>[2x]EIPLKYGATNEGKRQDPAMQKFRDNRLGAFIHWGLYAIPGGEWNGKVYGGAAEWLKSWAKVPADEWLKLMDQWNPTKFDAKKWAKMAKEM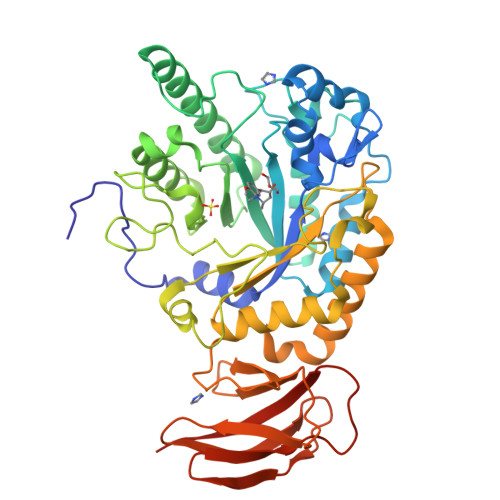GTKYVKITTKHHEGFCLWPSKYTKYTVANTPYKRDILGELVKAYNDEGIDVHFYFSVMDWSNPDYRYDIKSKEDSIAFSRFLEFTDNQLKELATRYPTVKDFWFDGTWDASVKKNGWWTAHAEQMLKELVPGVAINSRLRADDKGKRHFDSNGRLMGDYESGYERRLPDPVKDLKVTQWDWEACMTIPENQWGYHKDWSLSYVKTPIEVIDRIVHAVSMGGNMVVNFGPQADGDFRPEEKAMATAIGKWMNRYGKAVYACDYAGFEKQDWGYYTRGKNDEVYMVVFNQPYSERLIVKTPKGITVEKATLLTTGEDITVVETTRNEYNVSVPKKNPGEPYVIQLKVRAAKGTKSIYRDALT> GSMENLLEEVEKAKVIADEAVKLQKEIDKRCQHKIAEMVALMEKHKHQYDKIIEERDSELGLYKSKEQEQSSLRASLEIELSNLKAELLSVKKQLEI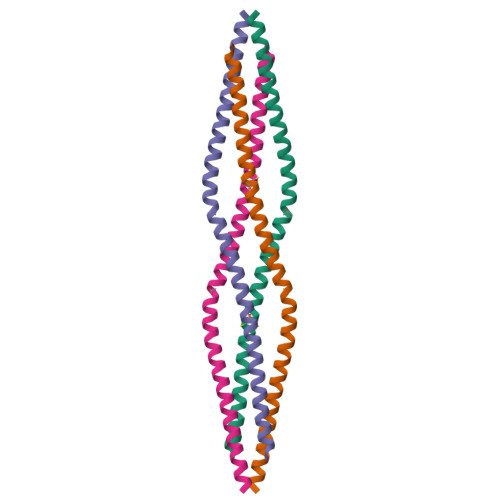E> GSGSAM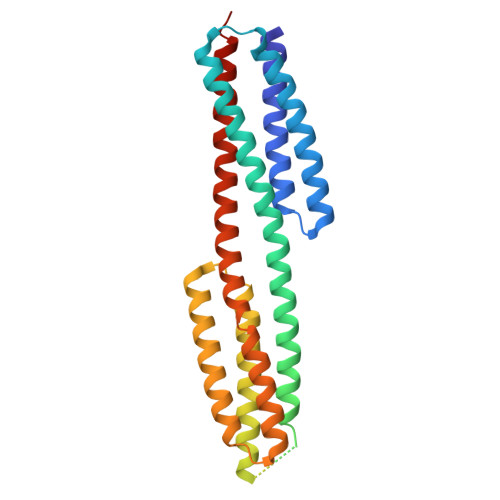IEARQVSELSTRIISSVQMLSNAQNEQERKEAGRVLFEQLESLLTHIKELGGESFDSKLLDALESNVQNVINNLAELGVTVERKLWLAKEIDTRVEEMRLLSEELEQLTRTQVQNTSTIAVANVTHIYDLLEANKKDQVYQALDALVEVDLDLTERLHELHLLAFKMLNQIEEARTLTNVDRIQQIQTAFENNLKIMKRRVLAVEDPTRSKQMSQLLTELGKRQVVFTILLQQYENNEQSQQLMQKTLELFSELNSTVNKLVDDSNKTTT>GSGSTRDYEIQRERIELGRCIGEGQFGDVHQGIYMSPENPALAVAIKTCKNCTSDSVREKFLQEALTMRQFDHPHIVKLIGVITENPVWIIMELCTLGELRSFLQVRKYSLDLASLILYAYQLSTALAYLESKRFVHRDIAARNVLV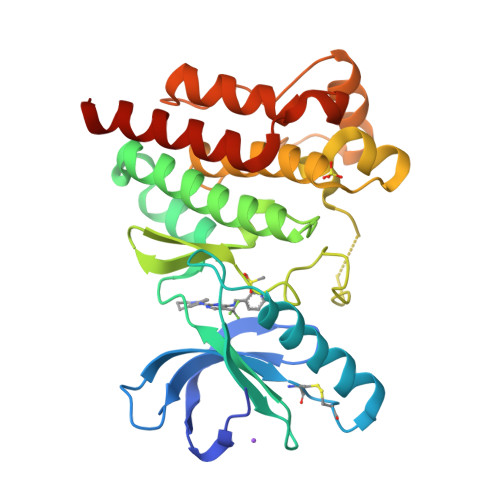SSNDCVKLGDFGLSRYMEDSTYYKASKGKLPIKWMAPESINFRRFTSASDVWMFGVCMWEILMHGVKPFQGVKNNDVIGRIENGERLPMPPNCPPTLYSLMTKCWAYDPSRRPRFTELKAQLSTILEEEKAQQEE[4x]> SNVEPVGRLHIFSGAHGPEKDFPLHLGKNVVGRMPDCSVALPFPSISKQHAEIEILAWDKAP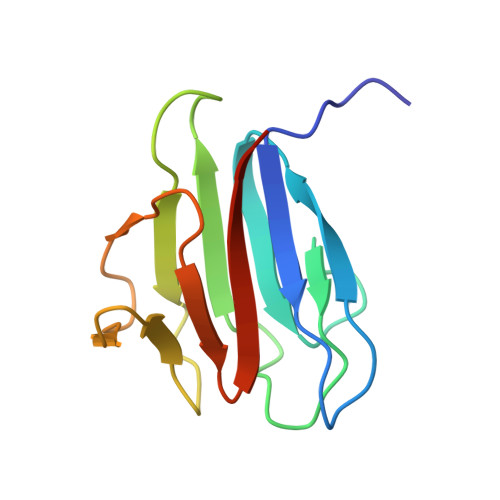ILRDCGSLNGTQILRPPKVLSPGVSHRLRDQELILFADLLCQYHRLDVSLP>MKTFAAYVIIACLSSTALAGSITENTSWNKEFSAEAVNGVFVLCKSSSKSCATNDLARASKEYLPASTFKIPNAIIGLETGVIKNEHQVFKWDGKPRAMKQWERDLTLRGAIQVSAVPVFQQIAREVGEVRMQKYLKKFSYGNQNISGGIDKFWLEGQLRISAVNQVEFLESLYLNKLSASKENQLIVKEALVTEAAPEYLVHSKTGFSGVGTESNPGVAWWVGWVEKETEVYFFAFNMDIDNESKLPLRKSIPTKIMESEGIIGG[2x]

Carbapenemases are the main cause of carbapenem resistance in Gram‐negative bacteria. How β‐lactamases with weak carbapenemase activity, such as the OXA‐10‐type class D β‐lactamases, contribute to anti‐bacterial drug resistance is unclear. OXA‐655 is a T26M and V117L OXA‐10 variant, recently identified from hospital wastewater. Here, we have solved crystal structures of OXA‐10 in complex with imipenem (IPM) and ETP, and OXA‐655 in complex with MEM in order to unravel the structure–function relationship and the impact of residue 117 in enzyme catalysis.

In summary, the crystal structures highlight the importance of residue 117 in OXA‐10 variants for carbapenemase activity. This study also illustrates the impact of a single amino acid substitution on the substrate profile of OXA‐10 and the evolutionary potential of new OXA‐10 variants.> LGASWHRPDKCCLGYQKRPLPQVLLSSWYPTSQLCSKPGVIFLTKRGRQVCADK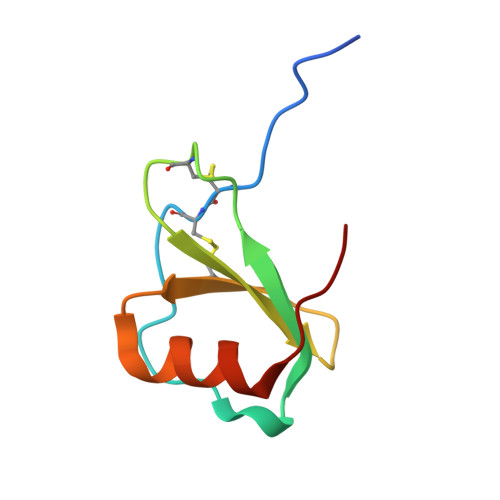SKDWVKKLMQQLPVTAR> MIADIDITAPEVLRNPYALFAELRRTSAVGRLQPQGFMAVGRYQDVARVLHDAKGFSNRGWAASLPRGVKWDTSMPPSIVQVDPPR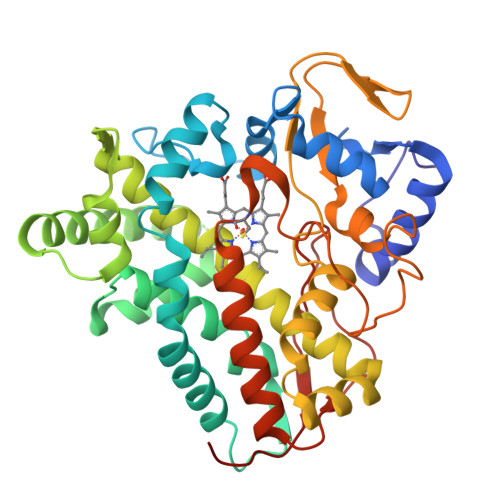HGKLRTLVTKAFTPRTVAQLEPRIRDIAHELVDGLRGKSTFEATVEVTVPMPMIVIAEMLGVAPERRADFKRWSDDMVGSLALVRVGNAAQLERSTQEFYAYFSEVLEERRREPREDLISQLLAAEVDGEKLTAGEVLSFANTLLIAGNETTTSLIGNALVALTDHPEQLAAAQADLSLVPAVVEEVLRYESPAQCIFRQTMTDVEIGDERIPARSVVLPLLASANRDESRFPDPDRFDIHRDTKGHLAFGLDIHFCIGAPLARLEAKVMLEVLLARLGDIQRVSQEVSWSPSFFIRSPSTLPLRATVASA> MHH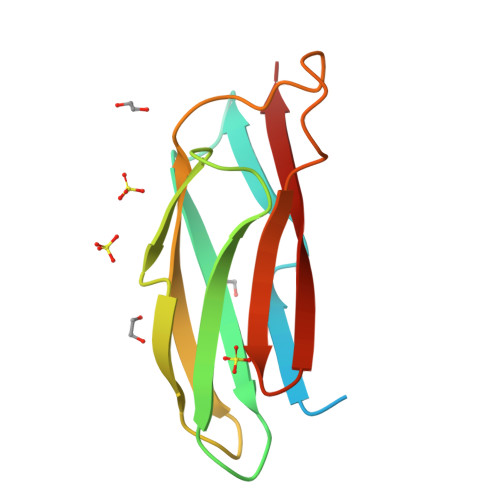HHHHSAGLEVLFQGPVEQNWCVQPGLLEFGVGCSPLATLSVTNSFCSRQLIEVTCNVPDLVRISPSECYVSPDGGHAEIDVRLLRSPRQDLLEREPLIVVSMENERISVPISFKF> SNAAGSLTSSRAKEVDISHLDPRMQQIVEKQITTAVKQYHAKSGVIAIADPQTGNIIAFAESSKNKGLESWKSRIFSPGSTIKPFIAAAAINSGNSSETKNYDCHSPYYIAGKTFTNYNSNVESASLADAIAKSINVCLIRVSQEAGVPVIRKKLTEFGFDMNSWWQADQSDDLQLAMAALGENIPVTIESLIKSYAILANKGHSFDRGNSAIISETSTNSINHMLENAVTNGTGKLAVIPGVSVAGKTGTVIENNDKYLALFAGYVPADNPRYVLLVVIEEGYFSKNGKTLVSGGELAAPVFRNVA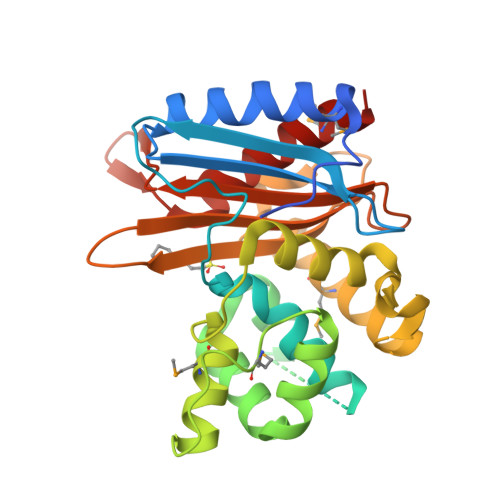MDALSSANR>SNAMKIVEVKHPLVKHKLGLMREHDISTKRFRELASEVGSLLTYEATADLETEKVTIEGWNGPVEVEQIKGKKITVVPILRAGLGMMEGVLEHVPSARISVVGIYRNEETLEPVPYFQKLVSNIDERMALVVDPMLATGGSMIATIDLLKNAGCTS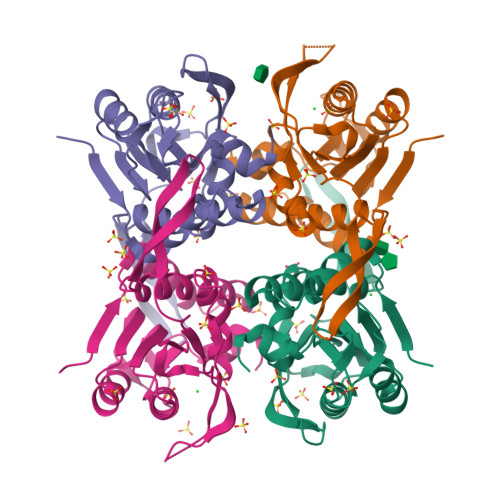IKVLVLVAAPEGIAALEKAHPDVELYTASVDKGLNEHGYIIPGLGDAGDKIFGTK[10x]>ACUCGUUUGAGCGAGUAUAAACAGUUGGUUAGGCUCAAAGCGGAGAGCAG[2x];>UCUGCUCUCXUCCAA[2x]

Small self‐cleaving ribozymes catalyze site‐specific cleavage of their own phosphodiester backbone. They are widely distributed in nature and are essential for rolling‐circle‐based replication of satellite and pathogenic RNAs. Comparative genomic analysis led to the discovery of novel self‐cleaving ribozymes, named twister, twister‐sister, pistol, and hatchet. In the present study we set out to obtain conformational snapshots along the reaction coordinate of the pistol ribozyme phosphordiester cleavage. We succeeded in solving the X‐ray structures of both its TS analogue vanadate (at 2.8 Å resolution) and the ternary 2′,3′ cyclophosphate product complex (at 2.65 Å resolution; see Figure S1 in the Suppporting Information for stereoviews).

To increase our understanding of the pistol ribozyme's catalytic mechanism, we have now determined its structure when complexed with a TS mimic at 2.8 Å resolution. To obtain the crystal structure of the TS analogue, we mixed the three RNA strands shown in Figure S2. The resulting complex lacks the scissile phosphate but retains the 2′‐, 3′‐, and 5′‐hydroxy groups at the cleavage site. This complex was co‐crystallized with NH4VO3. The electron density in the active site can be assigned to vanadate based on its size, shape, and anomalous scattering. Distances between the 2′‐, 3′‐, and 5′‐oxygen atoms and the vanadium atom are consistent with direct coordination between the oxygen atoms and the vanadium atom. Most importantly, while the key players (ribose‐32, G33, G40, G53, U54) in the active site only minimally alter their positions, the conformation of the backbone of the cleavage site is changed. The nonbridging oxygen centers of the scissile phosphate are rotated, bringing both the pro‐S oxygen and pro‐R oxygen centers much closer to the Hoogsteen face of G33 (shifting from 6.2 to 3.6 Å and from 4.4 to 3.3 Å towards N7‐G33, respectively). Furthermore, our TS analogue structure strongly suggests the bidentate interaction of G40 with the phosphorane TS during cleavage. In the vanadate complex both, N1 of G40 and N2 of G40 are within hydrogen‐bonding distance to the 2′O (2.5 Å) and the pro‐R oxygen atom (3.4 Å), respectively.>[3x]GSEFEPDEKEQKQLNQYAKTILFDTGKATIKFQSAEVLN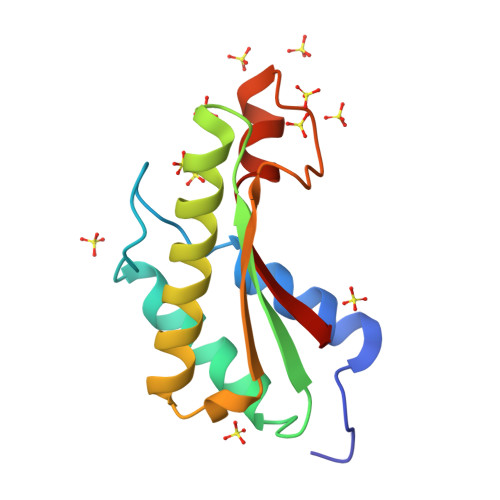QIINVLKKYPNSRFRIEGHTDSTGKKAKNMILSQNRADAVKVYLIQGGIDAGRLESQGFGPEKPIASNKNKKGRELNRRVEINLIK>GALSPGGTKQKYKEVVDIEAQRRLNDLAREARIRRAQQAVLRKELIATSTNVIKSEISLRILASECHLTLNGIVEAEAQYKMGGLPKSRLPKIKHP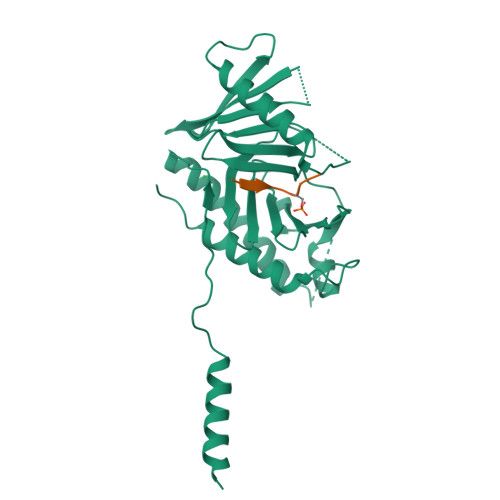MIVTKWVDYSNKHGFSYQLSTEDIGVLFNNGTTVLRLADAEEFWYISYDDREGWVASHYLLSEKPRELSRHLEVVDFFAKYMKANLSRVSTFGREEYHKDDVFLRRYTRYKPFVMFELSDGTFQFNFKDHHKMAISDGGKLVTYISPSHESTTYPLVEVLKYGEIPGYPESNFREKLTLIKEGLKQKSTIVTVD[2x];>[2x]SLAQSSPAGSQ7-(1H-imidazol-1-yl)-2-(pyridin-3-yl)[1,3]thiazolo[5,4-d]pyrimidin-5-amine | C13 H9 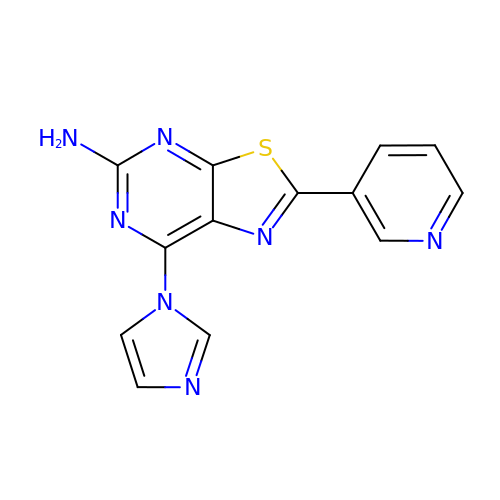N7 S | FTDVRDNCBWDKFI-UHFFFAOYSA-N>[4x]MGSSHHHHHHSSGLVPRGSRHSTLDFMLGAKADGETILKGLQSIFQEQGMAESVHTWQDHGYLATYTNKNGSFANLRIYPHGLVLLDLQSYDGDAQGKEEIDSILNKVEERMKELSQDSTGRVKRLPPIVRGGAIDRYWPTADGRLVEY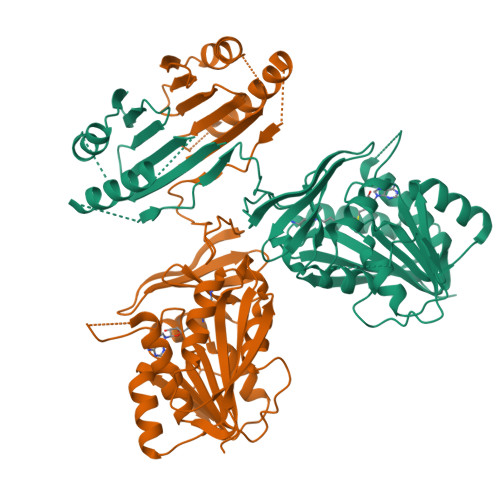DIDEVVYDEDSPYQNIKILHSKQFGNILILSGDVNLAESDLAYTRAIMGSGKEDYTGKDVLILGGGDGGILCEIVKLKPKMVTMVEIDQMVIDGCKKYMRKTCGDVLDNLKGDCYQVLIEDCIPVLKRYAKEGREFDYVINDLTAVPISTSPEEDSTWEFLRLILDLSMKVLKQDGKYFTQGNCVNLTEALSLYEEQLGRLYCPVEFSKEIVCVPSYLELWVFYTVWKKAKP> 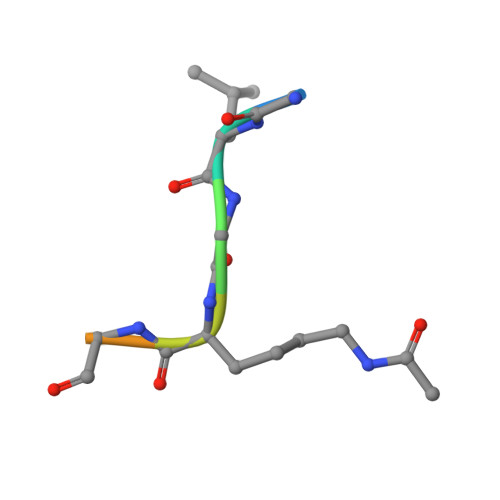GLGKGGAY Bacillus cereus (Bc) encodes three FNR paralogs, two of which have assigned distinct biological functions in bacillithiol disulfide reduction and flavodoxin (Fld) reduction. In this study, we have assigned a function to FNR1, in which the His residue is replaced by a conserved Val, in the reduction of the heme-degrading monooxygenase IsdG, ultimately facilitating the release of iron in an important iron acquisition pathway. The Bc IsdG structure was solved, and IsdG-FNR1 interactions were proposed through protein–protein docking. Mutational studies and bioinformatics analyses confirmed the importance of the conserved FAD-stacking residues on the respective reaction rates, proposing a division of FNRs into four functionally unique sequence similarity clusters likely related to the nature of this residue.

To investigate if the interchange of Val to His in FNR1 and His to Val in FNR2 could explain the differences in the efficiencies of Fld or IsdG reduction, we generated cross-mutants of the two proteins, FNR1V329H and FNR2H326V. For the FNR2H326V mutant, the λmax peak is shifted to a lower wavelength, while for FNR1V329H, it is shifted to a higher wavelength. In the case of FNR1V329H, replacing Val with His did not lead to an increase in the turnover number in the reduction of NrdI; on the contrary, we observed a kcat value 4-fold lower than for FNR1 and 55-fold lower than for FNR2. For Fld2, the turnover number using FNR1V329H as a reductase was shown to be 2-fold lower than with FNR1 and 480-fold lower than with FNR2. Although FNR1 has been previously shown to be a poorer reductase of Flds and NrdI than FNR2, these findings suggest that replacing the FAD-stacking Val residue for His in FNR1-type FNRs alone is not enough to make FNR1 a more efficient Fld reductase, somewhat distorting the fine-tuned chemical environment in the vicinity of the FAD cofactor. Comparing FNR1V329H to FNR1 as an IruO reveals that the FAD-stacking Val residue is a key structural feature important for the reduction of IsdG and breakdown of heme, as an approximately 2-fold slower rate of heme breakdown is observed using FNR1V329H as a reductase as compared to the wild-type enzyme. To investigate whether the altered reduction rates observed for the FNR2H326V and FNR1V329H mutants could be explained by their crystal structures, both structures were solved. The FNR1V329H structure is, with the exception of the mutation, highly similar to the wild-type FNR1 structure with an RMSD value of 0.2 Å. The mutation has not led to a change in the orientation of the NAD(P)H-binding domain relative to the FAD-binding domain, nor a movement of the other residues in the vicinity of the FAD cofactor. The lowered activity observed for FNR1V329H must therefore, from a structural perspective, be directly caused by the chemical properties of the single Val to His mutation, strengthening the importance of this residue for the biological function of FNR1.

>[2x]MNREELFDVTVIGGGPAGLYSAFYSGLREMRTKIIEFHPHLGGKIHVYPEKMIWDVGGLLPVTGDKLIEQLVQQGLTFKPEVVLDTKVESIIRNQDGTFTLKTSTGEEHFSKTVIVATGSGILKPQKLSIEGAERFEVSNLNYTVKSLKRFKGKTVIISGGGNSAVDWANELEPIAKKVYVTYRKEELSGHEAQVKQLMNSSAECFFNTSITKLIAGDNHEAIEYVELTNHETGEVSHLPIDEVIINHGYERDITLLENSELDVAIIDNYYIAGNANSESSVDGLYAAGDILKHEGKLHLIAGAFQDAGNAVNKAKQFIQPDASEYGMHSSHNEVFKKRNRELIKQMMK>SEKYDGEWNEGRMQGWGKYFYADGGVYEGEWVDGRMHGRGTYVFPNGNKYEGEWVEDRKDGYGILLYTNGERYEGYWHLDKAHGKGTLTFLQGDRYVGEWHYGKKHGHGVLSYSNGDTYDGEWRDDDAWGYGVLQYANGCRYEGEWAEDRRHGKGLLVLPDGSSYEGS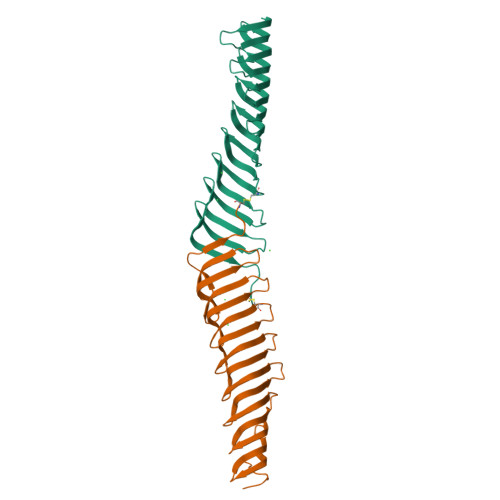FAHGKKDGPGKIILKDGSMYIGTWKDGVIVGQGEFRLSENCDLSNPDY[2x]> MPDTSFSNPGLFTPLQLGSLSLPNRVIMAPLTRSRTPDSVPGRLQQIYYGQRASAGLIISEATNISPTARGYVYTPGIWTDAQEAGWKGVVEAVHAKGGRIALQLWHVGRVSHELVQPDGQQPVAPSALKAEGAECFVEFEDGTAGLHPTSTPRALETDEIPGIVEDYRQAAQRAKRAGFDMVEVHAANACLPNQFLATGTNRRTDQYGGSIEN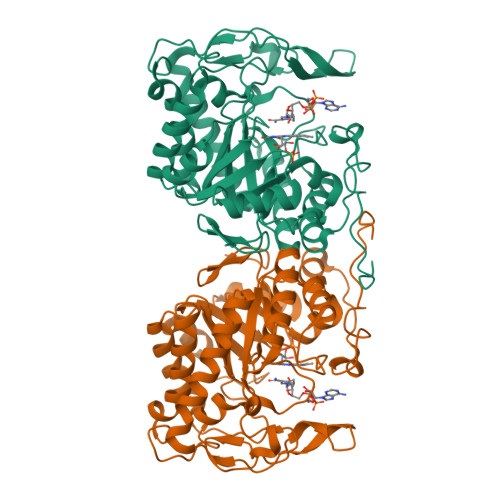RARFPLEVVDAVAEVFGPERVGIRLTPFLELFGLTDDEPEAMAFYLAGELDRRGLAYLHFNEPDWIGGDITYPEGFREQMRQRFKGGLIYCGNYDAGRAQARLDDNTADAVAFGRPFIANPDLPERFRLGAALNEPDPSTFYGGAEVGYTDYPFLDNGHDRLG> TRDQNGTWEMESNENFEGYMKALDIDFATRKIAVRLTQTKVIDQDGDNFKTKTTSTFRNYDVDFTVGVEFDEYTKSLDNRHVKALVTWEGDVLVCVQKGEKENRGWKQWIEGDKLYLELTCG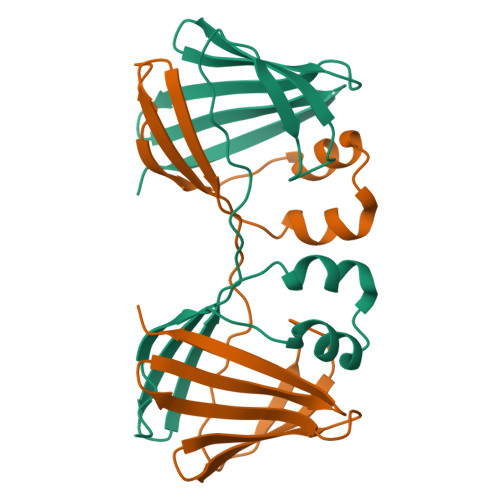DQVCRQVFKKK>GAPATVTEQGEDITSKKDRGVLKIVKRVGNGEETPMIGDKVYVHYKGKL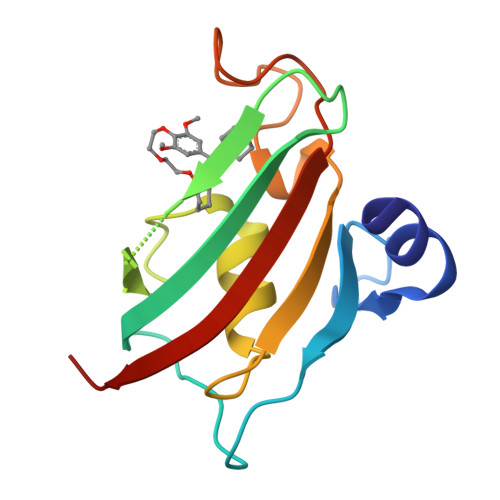SNGKKFDSSHDRNEPFVFSLGKGQVIKAWDIGVATMKKGEIAHLLIKPEYAYGSAGSLPKIPSNATLFFEIELLDFKGE[2x]>[2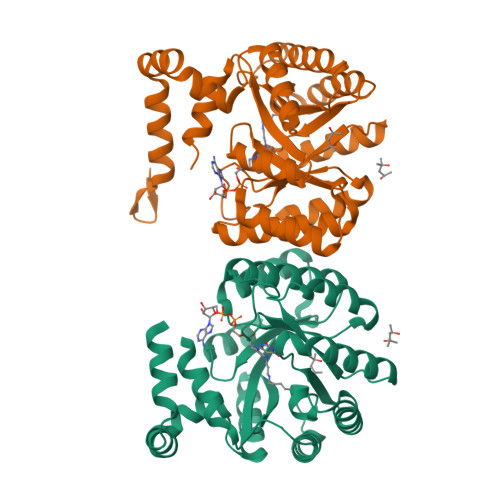x]MDHHHHHHHHASENLYFQGHMNLDLAYRSFVLGVAGHPQVERLIKHRAKGLVRRYVAGETLEEALKAAEALEREGVHAILDLLGEMVRTEEEARAFQRGLLELVWALAGKPWPKYISLKLTQLGLDLSEDLALALLREVLREAEPRGVFVRLDMEDSPRVEATLRLYRALREEGFSQVGIVLQSYLYRTEKDLLDLLPYRPNLRLVKGAYREPKEVAFPDKRLIDAEYLHLGKLALKEGLYVAFATHDPRIIAELKRYTEAMGIPRSRFEFQFLYGVRPEEQRRLAREGYTVRAYVPYGRDWYPYLTRRIAERPENLLLVLRSLVSG> MVKRTVATNGDASGAHRAKKMSKTHASHIINAQEDYKHMYLSVQPLDIFCWGTGSMCELGLGPLAKNKEVKRPRLNPFLPRDEAKIISFAVGGMHTLALDEESNVWSWGCNDVGALGRDTSNAKEQLKDMDADDSSDDEDGDLNELESTPAKIPRESFPPLAEGHKVVQLAATDNMSCALFSNGEVYAWGTFRCNEG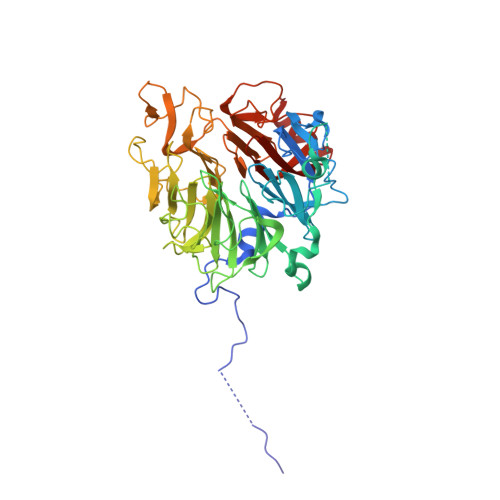ILGFYQDKIKIQKTPWKVPTFSKYNIVQLAPGKDHILFLDEEGMVFAWGNGQQNQLGRKVMERFRLKTLDPRPFGLRHVKYIASGENHCFALTKDNKLVSWGLNQFGQCGVSEDVEDGALVTKPKRLALPDNVVIRSIAAGEHHSLILSQDGDLYSCGRLDMFEVGIPKDNLPEYTYKDVHGKARAVPLPTKLNNVPKFKSVAAGSHHSVAVAQNGIAYSWGFGETYAVGLGPFEDDTEVPTRIKNTATQDHNIILVGCGGQFSVSGGVKLSDEDAEKRADEMDD(2S)-2-[(4R)-2-oxidanylidene-4-propyl-pyrrolidin-1-yl]butanamide | C11 H20 N2 O2 | 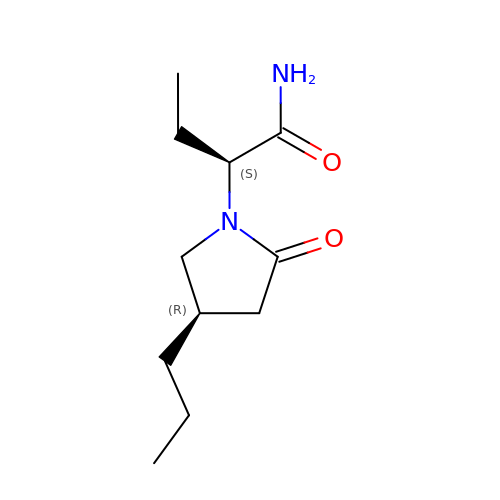MSYKRHVOOPPJKU-BDAKNGLRSA-N S-adenosyl-L-cysteine | C13 H18 N6 O5 S | 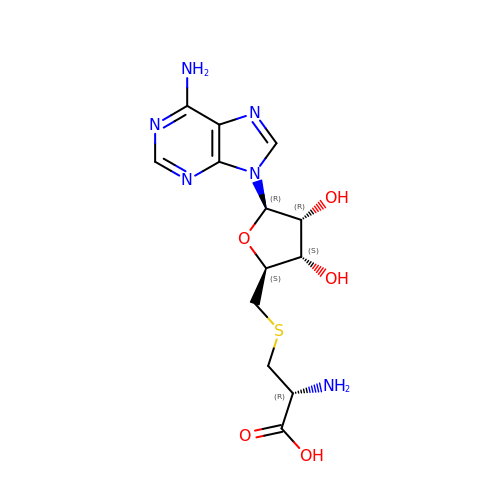RVFHZLGRQFCOKV-MACXSXHHSA-N> MGSSHHHHHHSSGENLYFQGHMGSGRVEVRVEFEGDKMRVRLRNDSSTPVEVHIKVGDEKRTVTVNPGEEVEVTFSANDPHKFNRPQFTIEWKDDKDGDGYISAAEKGRVEVRVEFEGDKMRVRLRNDSSTPVEVHIKVGDEKRTVTVNPGEEVEVTFSANDPHKFNRPQFTIEWG

Here, we devise geometrical principles for de novo designing single-chain immunoglobulin dimers, as a tunable two-domain architecture that optimizes biophysical properties through more favorable dimer interfaces. Here, we devise principles for de novo designing single-chain Ig dimers with interfaces diverging from Fvs, as a two-domain Ig architecture that is hard to find in nature and optimizes folding stability. We envisioned that de novo single-chain Ig dimers could be designed through two-layer edge-to-edge dimeric interfaces, resulting in extended Ig β-sandwiches. Key to such robustness is the two-layer edge-to-edge strand pairing at the interface between Ig domains, which involves a high number of backbone-backbone hydrogen bonds and protects oligomerization-prone β-sheet edges from solvent; overall favoring monomeric stability and solubility.

We computationally grafted an EF-hand calcium-binding motif (DKDGDGYISAAE; PDB 1NKF35) in the β-hairpin bridge of scIg12 (loop connecting both domains) by designing N- and C-terminal linkers (short and structured) to integrate the motif into the scaffold. Among the three most rigid designs identified by MD, we selected scIg12 + EF3a (loop sequence KDDKDGDGYISAAEK) for experimental characterization as it was the design with AlphaFold2 predictions of highest confidence (pLDDT > 90 for the five models and across all residue positions) and most similar to the design (Cα-RMSD < 1 Å). We also noted by MD that the structural rigidity of the binding motif increased in the presence of calcium and that the interactions of the four EF-hand binding residues (D71, D75, and E82 through their acidic sidechain and Y77 through the backbone oxygen atom) remained nearly constant throughout the simulation. We ordered a synthetic gene encoding for the design, and was found to be well-expressed in E. coli, soluble, and monomeric by SEC-MALS. Terbium-binding titrations were monitored at 544 nm with scIg12 + EF3a at 10 μM final concentration, and showed a hyperbolic increase in luminescence that was fitted to a 1:1 binding model, which gave an estimated Kd of 5.1 μM. Calcium was found to compete with terbium for the same binding site, but with much lower affinity (Kd = 1.3 mM)—this is expected given the lower charge density of calcium compared to terbium and hence weaker electrostatic interactions with the EF-hand motif. Lastly, we succeeded in solving the crystal structure of scIg12 + EF3a in a complex with terbium at 2.8 Å resolution by molecular replacement using the design model. The structure of the scaffold was found nearly identical to the design model (Cα-RMSD of 1.2 Å) and the parent scIg12 crystal structure (Cα-RMSD of 0.7 Å), which underscores the robustness of the extended β-sandwich scaffold to a 15-residue loop insertion.1-(4-fluorophenyl)-3-(3-hydroxyphenyl)urea | C13 H11 F N2 O2 | 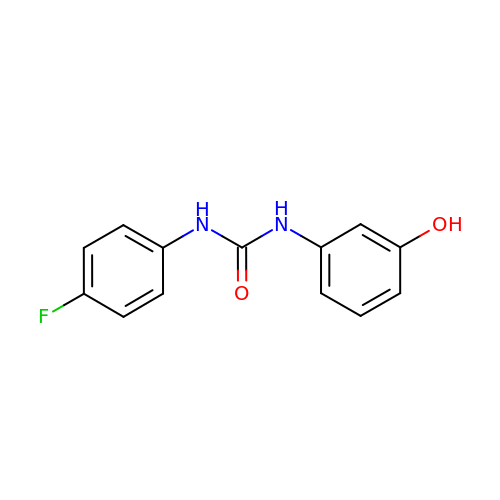BASVXNNPMBRKEP-UHFFFAOYSA-N> AEASADLRADAMAKDRSEEERTTEAEKNERVQKHLKALTSELANARDESK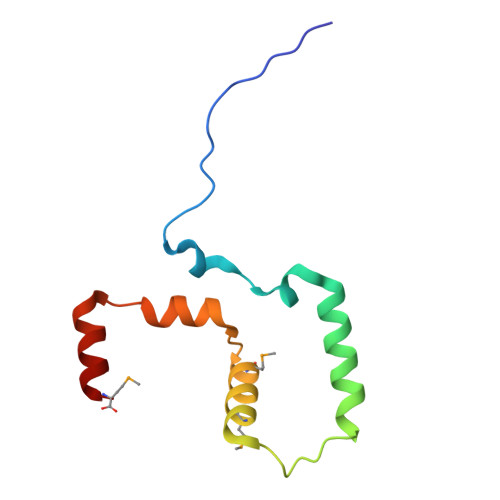KTANDMIHAENMRLGRDKYKTLRQIRQGNTKQRIDEFESM>[2x]MKKGHHHHHHGS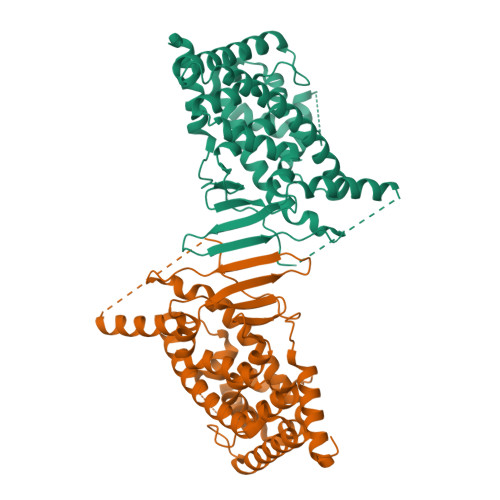ERTGTQPLGVQGLTEEQRMMIRELMDAQMKTFDTTFSHFKNFRLPGVLSSGCELPESLQAPSREEAAKWSQVRKDLCSLKVSLQLRGEDGSVWNYKPPADSGGKEIFSLLPHMADMSTYMFKGIISFAKVISYFRDLPIEDQISLLKGAAFELCQLRFNTVFNAETGTWECGRLSYCLEDTAGGFQQLLLEPMLKFHYMLKKLQLHEEEYVLMQAISLFSPDRPGVLQHRVVDQLQEQFAITLKSYIECNRPQPAHRFLFLKIMAMLTELRSINAQHTQRWLRIQDIHPFATPLMQELFGITGSSGGSGGSSHSSLTERHKILHRLLQEGSPSDITTLSVEPD> MAMPFEIEVLLPGELSPAETSALQKCEGKIITFSTLRHRASLVDIALSSYYINGAPPDTLSLLEAYRMRFAAVITRVIPGKLLAHAIGVGTPTPGLFIQNTSPVDLCNGDYICLLPPVFGSADSIRLDSVGLEIVFPLTIPQTLMREIIAKVVARAVERTAAGAQILPHEVLRGADVICYNGRRYELETNLQHRDGSDAAIRTLVLNLMFSINEGCLLLLALIPTLLVQGAHDGYVNLLIQTANCVRETGQLI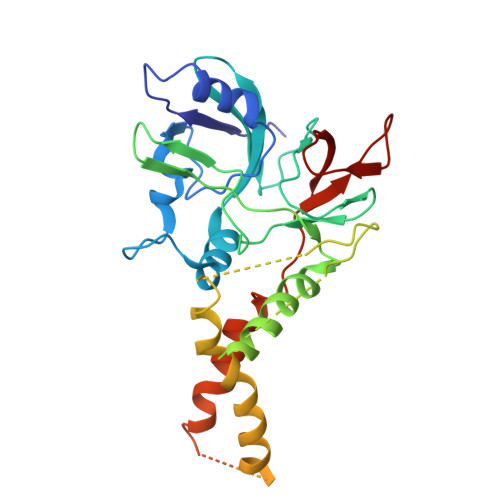NIPPMPRIQDGHRRFPIYETISSWISTSSRLGDTLGTRAILRVCVFDGPSTVHPGDRTAVIQV> GPSSPSAWNTNLRWRLPLTCLLLQVIMVILFGVFVRYDFEADAHWWSERTHKNLSDMENEFYYRYPSFQDVHVMVFVGFGFLMTFLQRYGFSAVGFNFLLAAFGIQWALLMQGWFHFLQDRYIVVGVENLINADFCVASVCVAFGAVLGKV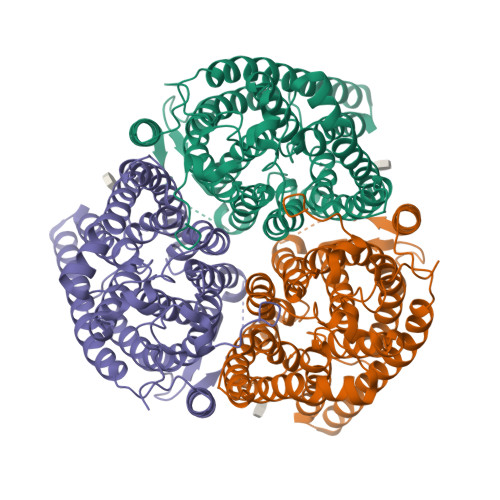SPIQLLIMTFFQVTLFAVNEFILLNLLKVKDAGGSMTIHTFGAYFGLTVTRILYRRNLEQSKERQNSVYQSDLFAMIGTLFLWMYWPSFNSAISYHGDSQHRAAINTYCSLAACVLTSVAISSALHKKGKLDMVHIQNATLAGGVAVGTAAEMMLMPYGALIIGFVCGIISTLGFVYLTPFLESRLHIQDTCGINNLHGIPGIIGGIVGAVTAASASLEVYGKEGLVHSFDFQGFNGDWTARTQGKFQIYGLLVTLAMALMGGIIVGLILRLPFWGQPSDENCFEDAVYWEMPEGNSTVYIPEDPTFKPSGPSVPSVPMVSPLPMASSVPLVPGGLVPR>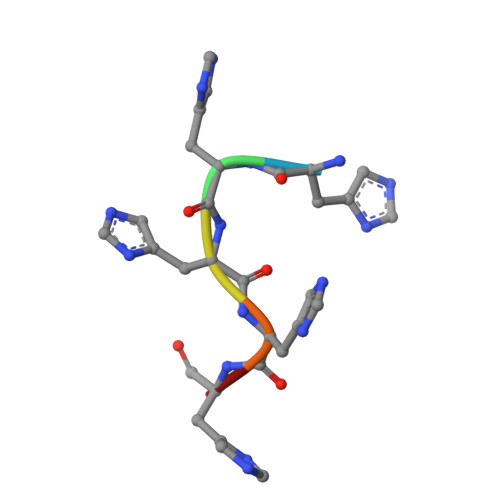 HHHHHH> MKNYARISCTSRYVPENCVTNHQLSEMMDTSAAWIHSRTGISERRIVTQENTSDLCHQVAKQLLEKSGKQASEIDFILVATVTPDFNM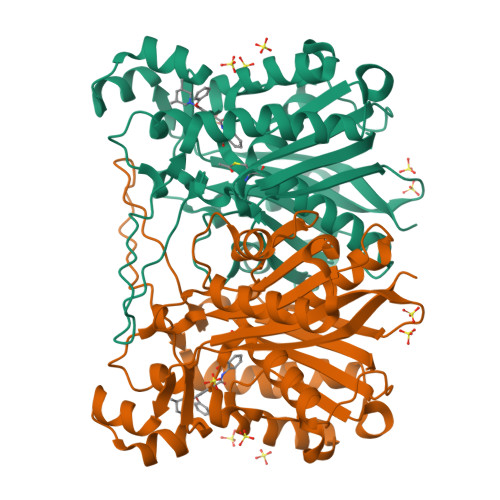PSVACQVQGAIGATEAFAFDISAACSGFVYALSMAEKLVLSGRYQTGLVIGGETFSKMLDWTDRSTAVLFGDGAAGVLIEAAETPHFLNEKLQADGQRWTALTSGYTINESPFYQGHKQASKTLQMEGRSIFDFAIKDVSQNILSLVTDETVDYLLLHQANVRIIDKIARKTKISREKFLTNMDKYGNTSAASIPILLDEAVENGTLILGSQQRVVLTGFGGGLTWGSLLLTL> MVVLAVLLPVVFGALLLLGLPRALGVLGAGLSFLLNLYLFLTHPGGVAHAFQAPLLPGAGVYWAFGLDGLSALFFLTIALTVFLGALVARVEGRFLGLALLMEGLLLGLFAARDLLVFYVFFEAALIPALLMLYLYGGEGRTRALYTFVLFTLVGSLPMLAAV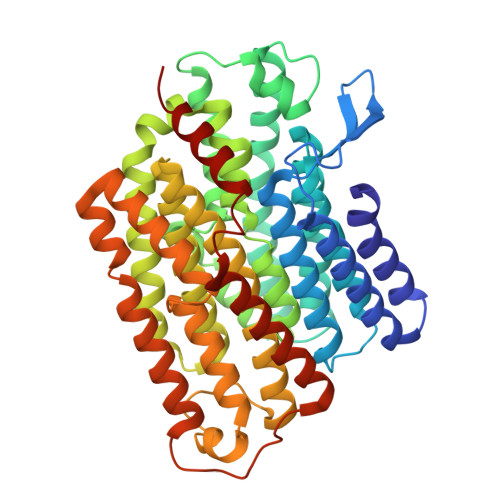LGARLLSGSPTFLLEDLLAHPLQEEAAFWVFLGFALAFAIKTPLFPLHAWLPPFHQENHPSGLADALGTLYKVGVFAFFRFAIPLAPEGFAQAQGLLLFLAALSALYGAWVAFAAKDFKTLLAYAGLSHMGVAALGVFSGTPEGAMGGLYLLAASGVYTGGLFLLAGRLYERTGTLEIGRYRGLAQSAPGLAALALILFLAMVGLPGLSGFPGEFLTLLGAYKASPWLAALAFLSVIASAAYALTAFQKTFWEEGGSGVKDLAGAEWGFALLSVLALLLMGVFPGYFARGLHPLAEAFAKLLGGGA> MSLGQSD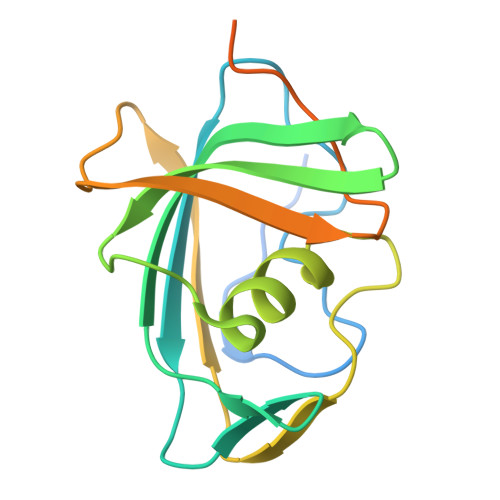LHIDPTQFIMYSGTISNGISYVNQAPSCGTVLSLKFTPGNSSLIENLHIEPYKVEVLKIEHVGDVSRATLLSDIVSLSTAQKKLLLYGFTQPGVQGLTGDVVSVETKRIPTPTQTNLLTIEDSIQCFTWDMNCANARSTNQDSRLIIYEQEDGRSHHHHHH>[4x]GPGTDFVYRVDSRPPEEIFRDGFRSHGFNRNLQQH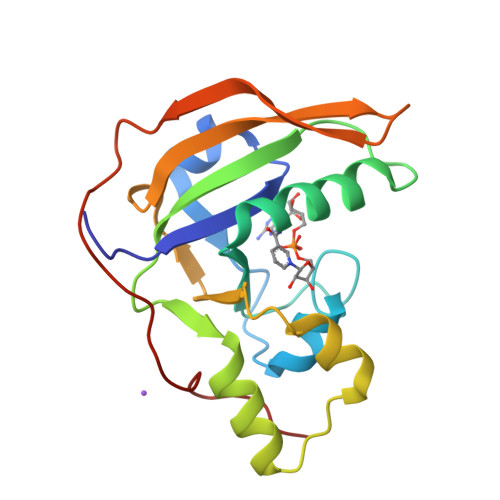LRGDSCAAGSRDSAFIATTTSLIETYNIARQYYSSSGFHGRLYRYRIRANNIFYPIQPSVNYLTQRGITFSGFERIMMREDNDIVAVEHIPGENIVEAVELTYDRFNSQVSDGPGTTNARYVPGSTFVNPGVIPQLVVPT> GAMGRNDNGAIRVYASSTIGNYILPEIIARYRRDFPDLPLEMSVGNSLDVVQAVCDFRVDIGLISGPCHMAEIVAQPWLEDELVVFASPASPLLEGEVTLERLAAMPWILREKGSGTREIVDYLLLSHLPQFRLSMELGNSEAIKHAVRHGLGVSCLSRRVIAEQLETGSLVEVKV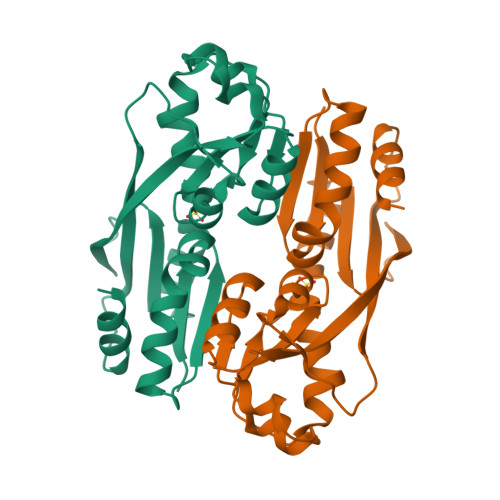PLPPLVRTLYRIHHRQKHLSSALARFLRYCEL>MRSRRVDVMDVMNRLILAMDLMNRDDALRVTGEVREYIDTVKIGYPLVLSEGMDIIAEFRKRFGCRIIADFKVADIPETNEKICRATFKAGADAIIVHGFPGADSVRACLNVAEEMGREVFLLTEMSHPGAEMFIQGAADEIARMGVDLGVKNYVGPSTAPERLSRLREIIGQDSFLISPGAGAQGGDPGE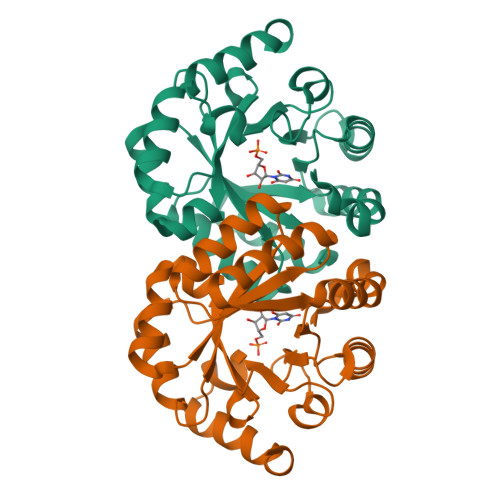TLRFADAIIVGRSIYLADNPAAAAAGIIESIKDLLNP[2x]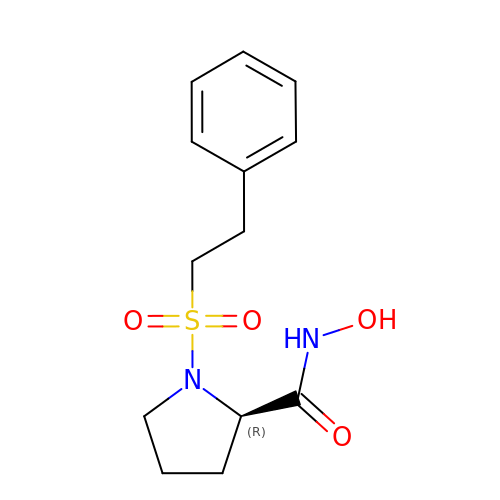N-hydroxy-1-[(2-phenylethyl)sulfonyl]-D-prolinamide | C13 H18 N2 O4 S | FTQOZDRDOVWSBK-GFCCVEGCSA-N> HPETLVKVKDAEDQLGARVGYIELDLNSGKILESFRPEERFPMMSTFKVLLCGAVLSRVDAGQEQLGRRIHYSQNDLVEYSPVTEKHLTDGMTVRELCSAA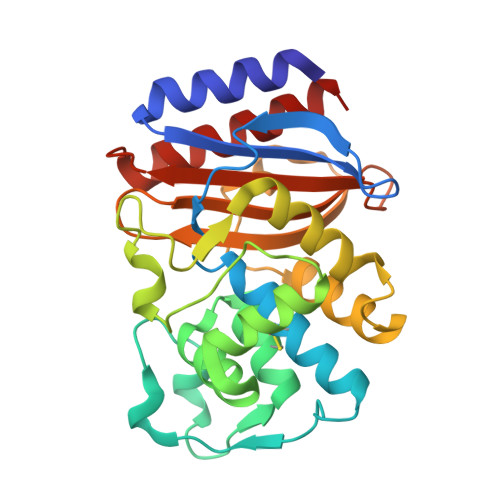ITMSDNTAANLLLTTIGGPKELTAFLHNMGDHVTRLDRWEPELNEAIPNDERDTTMPAAMATTLRKLLTGELLTLASRQQLIDWMEADKVAGPLLRSALPAGWFIADKSGAGERGSRGIIAALGPDGKPSRIVVIYTTGSQATMDERNRQIAEIGASLIKHW> MHHHHHHIEGRQYKDGYYITTLNYNFNTVYNATLQAIQNGQTFDYKSNPYDISVNKNNGTDAEIVSASDSDSTDSLQVAMKKLPNNATRISIKYGSQGNSIRSSALIG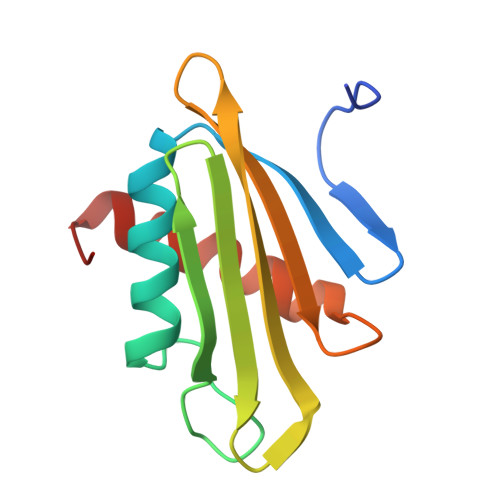IIEGNIRYANT> PNSMKNIESLFDYSAGQFEFIDHLLTMGVGVHFAALIFFLVVSQFVAPKYRIATALSCIVMVSAGLILNSQAVMWTDAYAYVDGSYQLQDLTFSNGYRYVNWMATIPCLLLQLLIVLNLKGKELFSTATWLILAAWGMIITGYVGQLYEVDDIAQLMIWGAVSTAFFVVMNWIVGTKIFKNRATMLGGTDSTITKVFWLMMFAWTLYPIAYLVPAFMNNADGVVLRQLLFTIADISSKVIYGLMITYIAIQQSAAAGYVPAQQALGRIGMDSKAA

In contrast, the NTQ rhodopsin functions as a light-driven inward chloride pump (called ClR). Here we report the atomic crystal structure of ClR from the flavobacterium Nonlabens marinus S1-08T. The structure reveals two chloride ion-binding sites, one at the active centre of the pump and the other on a loop in the cytoplasmic side, suggesting the pathway of chloride ion movement in ClR. The ClR structure comprises a short N-terminal helix, seven transmembrane helices (TM A–TM G), a C-terminal helix and three loops connecting the transmembrane helices on both extracellular and cytosolic sides.

We crystallized ClR from N. marinus under two different sets of conditions using the lipid cubic phase method. Type A crystals, obtained at pH 6.0, diffracted to 1.56 Å and type B crystals, obtained at pH 4.5, diffracted to 2.0 Å. The type A and type B crystal structures were refined to a Rwork/Rfree of 15.40/19.38% and 17.84/22.24%, respectively. The final type A and type B crystal structures contained ClR residues 2–265 and 1–266, respectively. The retinal adopts the all-trans conformation in the ClR structure. Cl−-I, which is located 3.1 Å away from PSB, interacts directly with PSB by electrostatic and hydrogen-bonding interactions. The conserved Asn98 and Thr102 of the NTQ motif are hydrogen bonded with Cl−-I, stabilizing the coordination of Cl−-I. Three water molecules (W501, W502 and W503) that interact with amino-acid residues are well resolved around Cl−-I and PSB. In the crystal structure, ClR adopts a conformation in which the extracellular side is open to the solvent area, whereas the cytosolic side is occluded from the solvent area. Water molecules inside the ClR structure indicate the presence of three internal cavities (IC1, IC2 and IC3). The C-terminal helix of ClR is also amphipathic and its hydrophobic interface, formed by Pro257, Ala258, Ala261, Leu262 and Ile265, interacts with an oleic acid located on TM A.> MPIHHHHHHQHNLKTSVVESREQRLGTIIAWDGKASDLSKESAYARSEGCGSACGAKARRVCEMRSPFSQGSVCSEQMVECQAGNVRGAVLVQHSPIGCGAGQVIYNSIFRNGLAIRGLPVENLHLISTNLRERDMVYGGLDKLERTIRDAWERHHPQAIFIATSCPTAIIGDDIESVASQLEAEFGIPVIPLHCEGFKSKHWSTGFDATQHGILRQIVRKNPERKQEDLVNVINLWGSDVFGPMLGELGLRVNYVVDLATVEDLAQMSEAAATVGFCYTLSTYMAAALEQEFGVPEVKAPMPYGFAGTDAWLREIARVTHREEQAEAYIAREHARVKPQLEALREKLKGIKGFVSTGSAYAHGMIQVLRELGVTVDGSLVFHHDPVYDSQDPRQDSLAHLVDNYGDVGHFSVGNRQQFQFYGLLQRVKPDFIIIRHNGLAPLASRLGIPAIPLGDE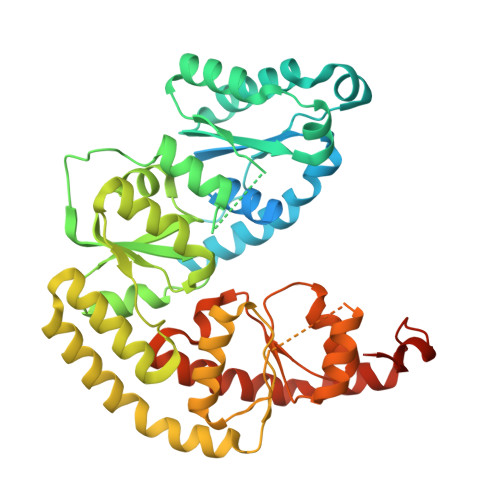HIAVGYQGILNLGESILDVLAHRKFHEDIAAHVRLPYRQDWLARDPFDLARQSAGQPRRPAE>UGGAAGAAAUCGAAGAAGAUGAAGAACGCGAAGAAC[2x];>AUCUUCUUCGAUUUCUUCCAGUUCU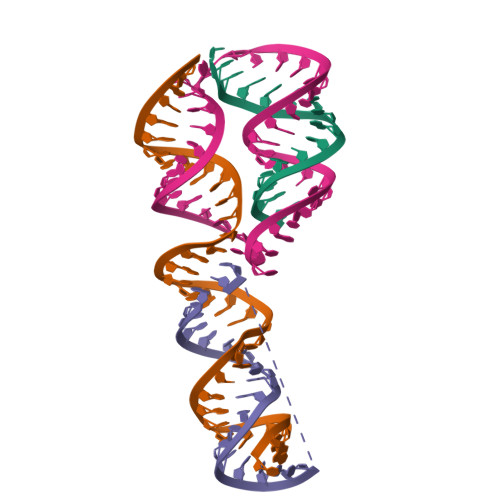UCGCGUUCUUC[2x]> KFE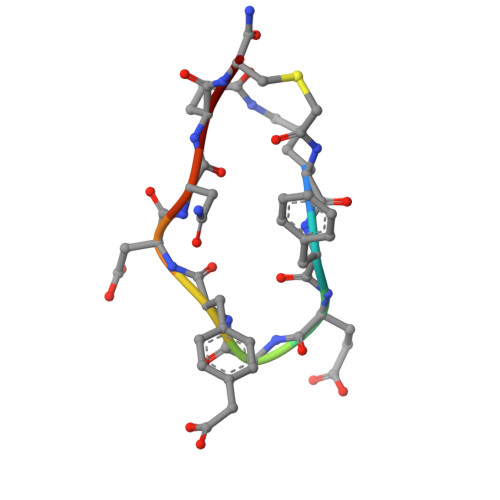GFDNEX> MRVFHFSKLPLGVAILAASSSVFAVTLDGGAVAAPDQYGAKVAAEILKKGGNAVDAAVATAFTLAVTYPEAGNIGGGGFMTLYVDGKPYFLDYREIAPKAATKTMYLNEKGEVIENLSLVGAKAAGVPGTVMGLWEAHQRFGKLKWSELLTPAIGYAQTGFKVADQQYQYRQDAIALFNGKTNFGDYFGTMKPGEVFKQPELAKTLERIADKGPDDFYKGETAKLLIAQMKQDGGLITSDDLVDYQAKWREPMRIDWQGNTLYTAPLPSSGGIALAQ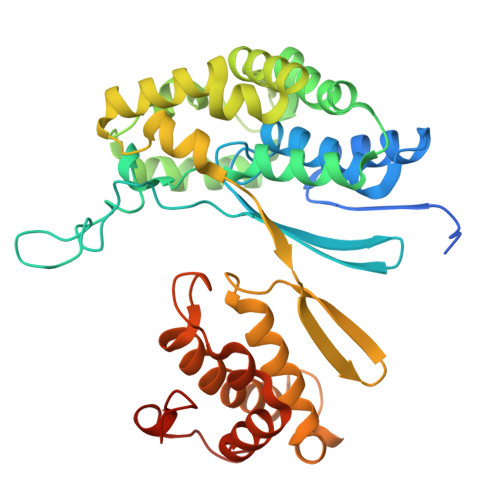LIGIKEQRAADFKGVELNSAKYIHLLSEIEKRVFADRADYLGDPQFSKVPVAQLTDPKYIAKRAGEVNPDAISATEKVRPGLEPHQTTHFSIVD> DKMNSVG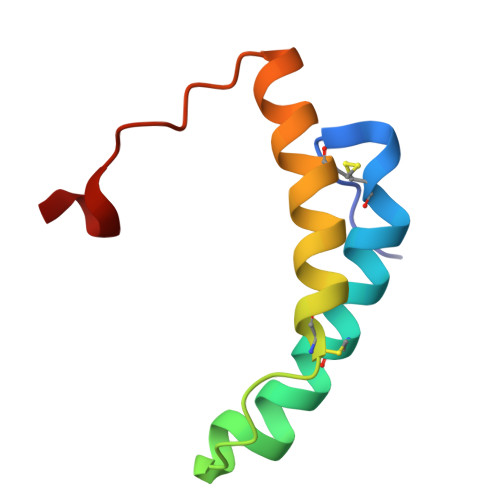EACTDMKREYDQCFNRWFAEKFLKGDSSGDPCTDLFKRYQQCVQKAIKEKEIPIEGLEFMGH>MGPSLDFALSLLRRNVRQVQTDQGHFTMLGV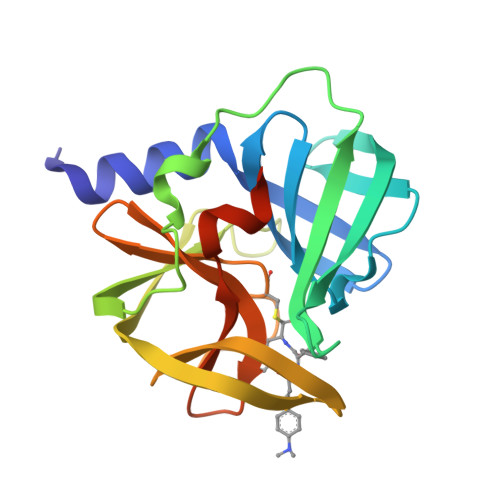RDRLAVLPRHSQPGKTIWIEHKLVNILDAVELVDEQGVNLELTLITLDTNEKFRDITKFIPENISTASDATLVINTEHMPSMFVPVGDVVQYGFLNLSGKPTHRTMMYNFPTKAGQCGGVVTSVGKVIGIHIGGNGRQGFCAGLKRSYFASEQLEHHHHHH[2x]> SNAMSKQLLALNIDGALLRSNGKIHQATKDAIEYVKKKGI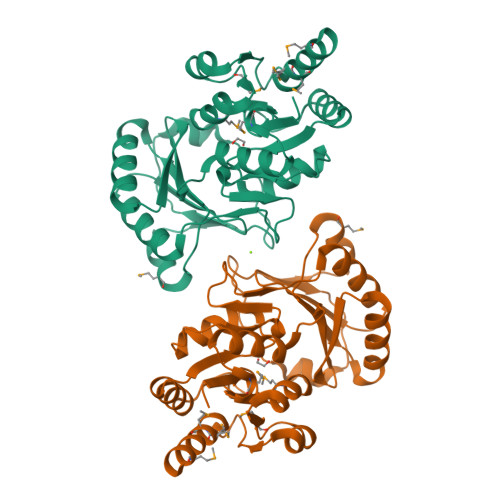YVTLVTNRHFRSAQKIAKSLKLDAKLITHSGAYIAEKIDAPFFEKRISDDHTFNIVQVLESYQCNIRLLHEKYSIGNKKKVNSNLLGKALIHPSDPIFYPVQFVESLSDLLMDEPVSAPVIEVYTEHDIQHDITETITKAFPAVDVIRVNDEKLNIVPKGVSKEAGLALVASELGLSMDDVVAIGHQYDDLPMIELAGLGVAMGNAVPEIKRKADWVTRSNDEQGVAYMMKEYFRMQQRKGFLDKFHMKR> GSHMKNSVSVDLPGSMKVLVSKSSNADGKYDLIATVDALELSGTSDKNNGSGVLEGVKADASKVKLTISDDLGQTTLEVFKSDGSTLVSKKVTSKDKSSTEEKFNEKGEVSEKIITRADGTRLEYTGIKSDGSGKAKEVLKGYVLEG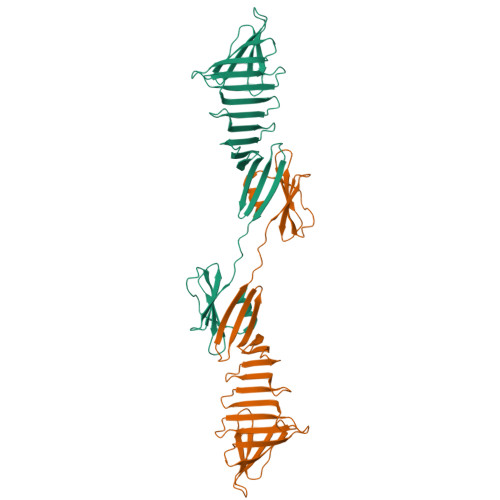TLTAEKTTLVVKEGTVTLSKNISKSGAVSVELNDTPPPPPKKTAAWNSGTSTLTITVNSKKTKDLVFTSSNTITVQQYDSNGTSLEGSAVEITKLDEIKNALK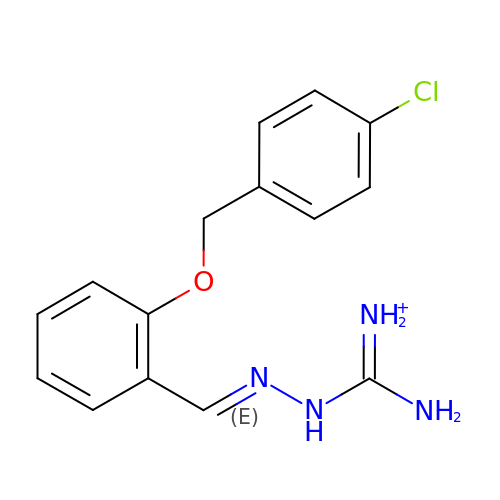[azanyl-[(2E)-2-[[2-[(4-chlorophenyl)methoxy]phenyl]methylidene]hydrazinyl]methylidene]azanium | C15 H16 Cl N4 O | QLZIJPLTRJOVDN-DJKKODMXSA-O2-{5-[AMINO(IMINIO)METHYL]-6-FLUORO-1H-BENZIMIDAZOL-2-YL}-6-ISOBUTOXYBENZENOLATE | C18 H19 F N4 O2 | 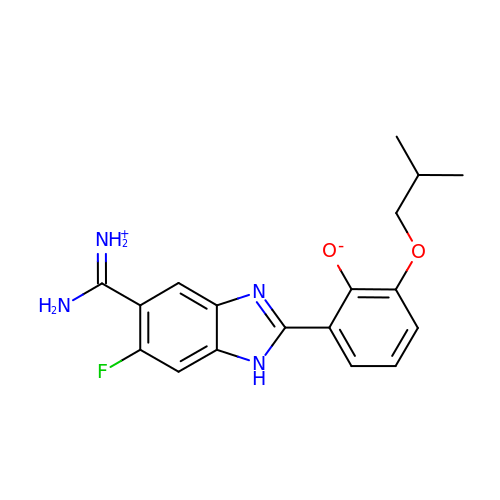NSUDDASMRZSVON-UHFFFAOYSA-N>MHKRTLLFKNAELLVTMDDERREIRGGCLLVEGNRIVAVGGDELCAAPADEEIDLRGHIVIPGLINTHHHMFQSLTRVIPDAQDGELFDWLNNLYPIWAGLTPEMIRISTQTAMAELMLSGCTTSSDHLYVYPNGCRLDDSIDGAREIGMRFHACRGSMSVGRSKGGLPPDELVENEQAILEDSLRLIHSYHDAQRYSMLRIALAPCSPFSVSRELMVKTAQMAREQGVSLHTHLAENDSDVSYSQTHFGMTPAQYAEDLGWVGSDVWHAHCVKLDRAGISLFAR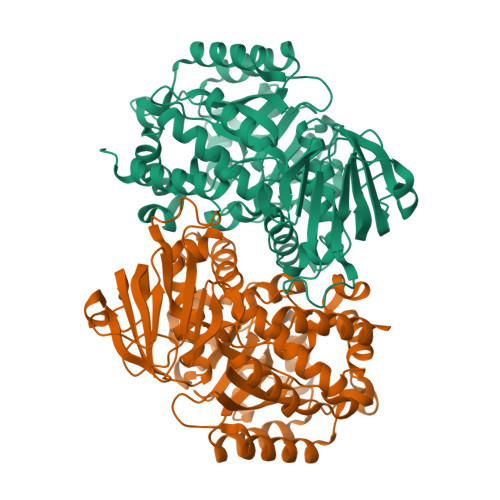TGTGVAHCPCSNMRLASGIAPIRAMLDEGVSVGLGVDGSASNDAGNMIAETRQAMLLQRVGFGPDAMNARQALEIATRGGAKVLNRDDIGYLATGMAADFVAFDLNTLNLAGAKHDPLAALVFCTPGNVAFSVINGQVVIREGVLQTIDLPSVVQQHNRLACLLVNRHRL[2x]>MTTPFMSNMTGWTTVNGTWADTIEGKQGRSDGDSFILSSASGSDFTYESDITIKDGNGRGAGALMFRSDKDAKNGYLANVDAKHDLVKFFKFENGAASVIAEYKTPIDVNKKYHLKTEAEGDRFKIYLDDRLVIDAHDSVFSEGQFGLNVWDATA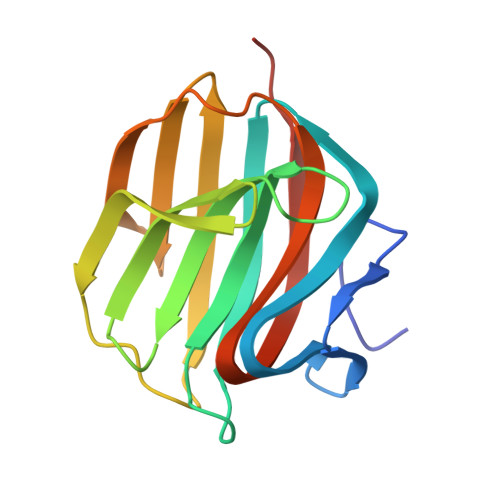VFQNVTKESLEHHHHHH[2x]5-METHYL-2-[(PHENYLSULFONYL)AMINO]BENZOIC ACID | C14 H13 N 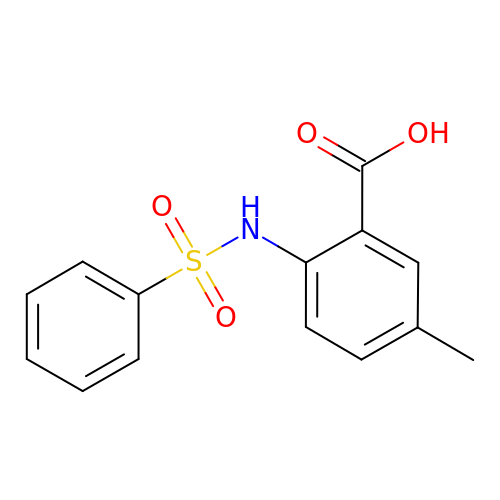O4 S | HXQLTRSIZRSFTR-UHFFFAOYSA-N> MATVEPETTPTPNPPTTEEEKTESNQEVANPEHYIKHPLQNRWALWFFKKDKSKTWQANLRLISKFDTVEDFWALYNHIQLSSNLMPGCDYSLFKDGIEPMWEDEKNKRGGRWLITLNKQQRRSDLDRFWLETLLCLIGESFDDYSDDVCGAVVNVRAKGDKIAIWTTECENREAVTHIGRVYKERLGLPPKI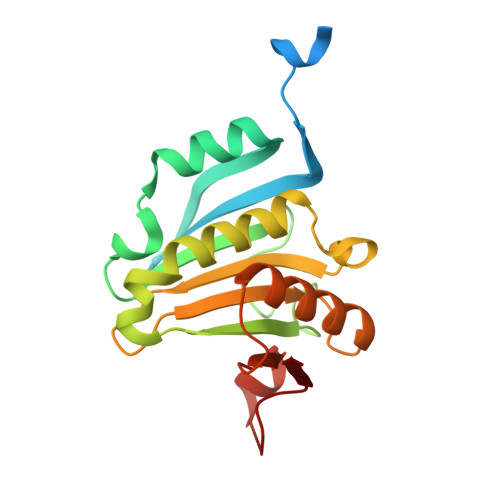VIGYQSHADTATKSGSTTKNRFVV>[2x]MGSVTCTGCVDLDELSFEKTVERFPYSVVKFDIAYPYGEKHEAFTAFSKSA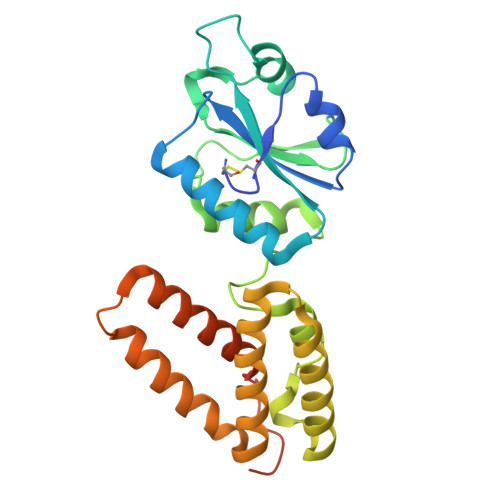HKATKDLLIATVGVKDYGELENKALGDRYKVDDKNFPSIFLFKGNADEYVQLPSHVDVTLDNLKAFVSANTPLYIGRDGCIKEFNEVLKNYANIPDAEQLKLIEKLQAKQEQLTDPEQQQNARAYLIYMRKIHEVGYDFLEEETKRLLRLKAGKVTEAKKEELLRKLNILEVFRVHKVTKTAPEKEELRGSHHHHHH1-deoxy-L-erythrulose | C4 H8 O3 | 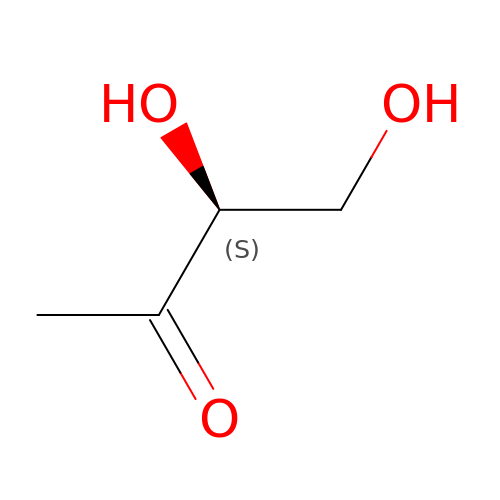SEYLPRWNVFCVRQ-BYPYZUCNSA-N(5~{S})-1-methyl-5-pyridin-3-yl-pyrrolidin-2-one | 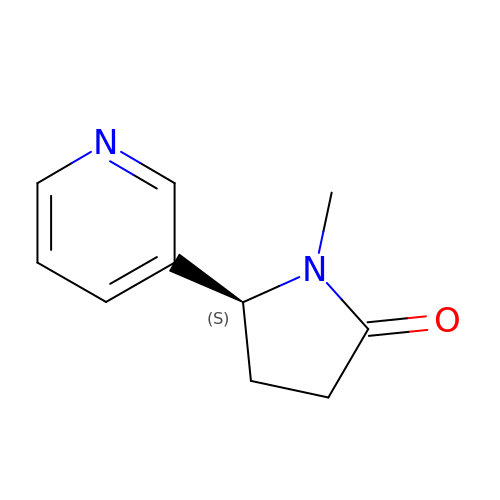C10 H12 N2 O | UIKROCXWUNQSPJ-VIFPVBQESA-N> FSPQLLSLLSLKTSLSGPPSAFQDWKVPVNGQNDAVWCSWSGVVCDNVTAQVISLDLSHRNLSGRIPIQIRYLSSLLYLNLSGNSLEGSFPTSIFDLTKLTTLDISRNSFDSSFPPGISKLKFLKVFNAFSNNFEGLLPSDVSRLRFLEELNFGGSYFEGEIPAAYGG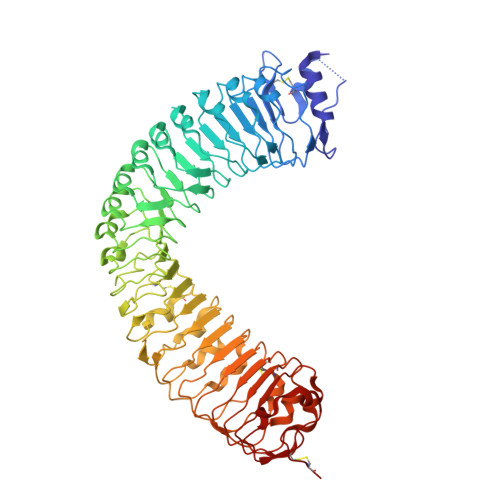LQRLKFIHLAGNVLGGKLPPRLGLLTELQHMEIGYNHFNGNIPSEFALLSNLKYFDVSNCSLSGSLPQELGNLSNLETLFLFQNGFTGEIPESYSNLKSLKLLDFSSNQLSGSIPSGFSTLKNLTWLSLISNNLSGEVPEGIGELPELTTLFLWNNNFTGVLPHKLGSNGKLETMDVSNNSFTGTIPSSLCHGNKLYKLILFSNMFEGELPKSLTRCESLWRFRSQNNRLNGTIPIGFGSLRNLTFVDLSNNRFTDQIPADFATAPVLQYLNLSTNFFHRKLPENIWKAPNLQIFSASFSNLIGEIPNYVGCKSFYRIELQGNSLNGTIPWDIGHCEKLLCLNLSQNHLNGIIPWEISTLPSIADVDLSHNLLTGTIPSDFGSSKTITTFNVSYNQLIGPIPSGSFAHLNPSFFSSNEGLCGDLVGKPCN> GATQGTADKDAQITQDWSVEKLYAEAQDELNSSNYTRAVKLYEI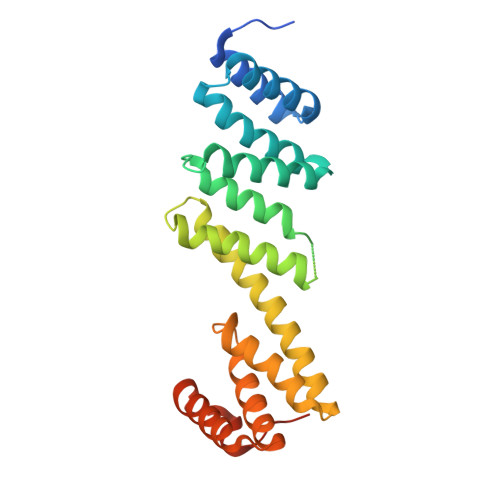LESRFPTSRHARQSQLDTAYAYYKDDEKDKALAAIERFRRLHPQHPNMDYALYLRGLVLFNEDQSFLNKLASQDWSDRDPKANREAYQAFAELVQRFPNSKYAADATARMVKLVDALGGNEMSVARYYMKRGAYIAAANRAKKIIGSYQNTRYVEESLAILELAYKKLDKPQLAADTRRVLETNFPKSPFLTHAWQPDDMPWWRYWH> MYAYNGKLLDVDLTREKVKEVELSEDVLKKFYGGRGL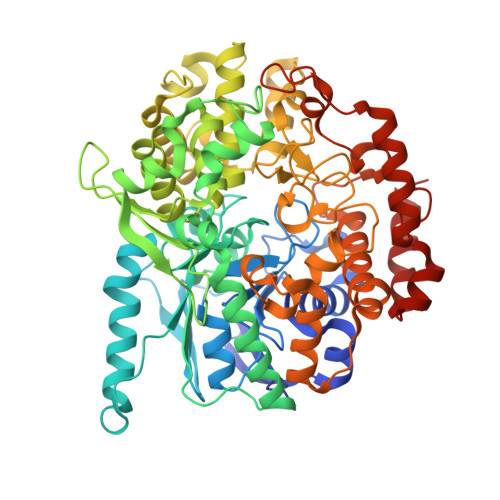GTYILWKELGEKWEKVDPLGEENLLLILTGPLTGYYPGMKTSIVSKSPESNGVVGSVLSSELGLELKAAGYDGIIIRGKAKSPVYLFIHNDTVEIRDATKYWGMGGIELYKTLLKEVHEEIRKKEKLKGVPKEPAMIYIGKGGENKVRFAAIMTKLMHAAGYGGYGAVMGSKNLKAVIAKGSGPLPEVYDKEKMKVLLREFWKELFSMTTFREWGTGAGGYSVGHDRSSEPIRNWQEEYHDNEEISVVNFENRTWIKKYWADYGCPVNCMKISYLRYGPYKGSISDAPDYELQAYMGTNLGIFEPEKIVYLSYLVDELGLDGINTGNILGFAAELYQRGILTKEDLGFELNWGDEKAFAKLLHLIVEKEGIGKILAEGTYRAALKISEIKGIDVTKYAVHVKGIAVGAHGIRSELDYTKDISYAVSVQGGDHTSTAALPAKGYTGELVEAFYDSAVICNFVTKPGFEKIIEFGNALSGFNITPEQWLNEIGLRIIHLQRILLLLGGPDVYWDPRKDDDNPPRFYEPLPSGPVKGKAPNREDIKAKVKQYYEEIGYDEHGIPKEEVLEELGIGEAKREVKRIKKRLNL The bacterial General Secretory System is centred around two essential components: the SecYEG complex, which forms a pore through the cytoplasmic membrane, and SecA, an ATPase that couples ATP binding and hydrolysis to translocation of an unfolded preprotein substrate through the SecYEG pore. Attempts to address this question have been confounded by the fact that SecA exists as a dimer in solution, but given the changes in SecA oligomerization required for its interaction with SecYEG, it is not clear whether the solution dimer is related to oligomeric species that may participate in the translocation reaction. Truncation of E. coli SecA at residue 610 produces a construct, SecA-N68, that is monomeric at low concentrations but at higher concentrations forms tetramers. In the current work, we have discovered that the formation of the SecA-N68 tetramer is completely dependent on unstructured polypeptide segments at its N- and C-termini.

To obtain a structure of the E. coli PPXD, we used a deletion construct, “SecA-N68” that lacks the C-terminal domains, including the Helical Wing Domain (HWD), the Helical Scaffold Domain (HSD), and a linker connected to the Zinc Binding Domain (ZBD). To obtain crystals of SecA-N68, we removed unstructured regions at the N- and C-termini so that the construct included residues 15 to 590, which we term “SecA-N68∆NC”. In addition, entropy-reducing mutations to alanine37 were introduced in two areas, one containing E55, K56, and E58, and a second at E196 and E197. In addition, removal of the termini allowed us to obtain crystals of SecA-N68 that diffracted to 2.6 Å resolution and yielded a structure that includes both the DEAD Motor domains and the preprotein crosslinking domain (PPXD), which was disordered in the original E. coli SecA structure. The structure of SecA-N68∆NC bound to Mg2+-ADP contains the DEAD Motor domains, NBD1 and NBD2, in the same conformation observed for other SecA structures, with the exception of the E. coli SecA structure which was crystallized in the absence of bound nucleotide and in which NBD1 and NBD2 adopt a more open conformation. The β-hairpin anchoring the PPXD to NBD1 is in a fully extended conformation that has not been observed in previous crystal structures, where the hairpin is typically bent to facilitate interaction of the PPXD with the C-terminal helical domains. The core PPXD structures are conserved throughout, with some differences in loop regions. Helix 4 is particularly well-conserved, likely because it plays a central role, interacting directly with SecYEG as well as Helix 1, 3, and Hairpin 2. That is, SecA-N68∆NC, in which both N- and C-termini had been truncated to remove unstructured polypeptide but is otherwise identical to SecA-N68, is completely monomeric when analyzed by gel filtration chromatography. Formation of the SecA-N68 tetramer is completely dependent on unstructured polypeptide at the N- and C-termini.

> GADRTLRRMRKVVNIINAMEPEMEKLSDEELKGKTAEFRARLAAGAVLENLIPEAFAVVREASKRVFGMRHFDVQLLGGMVLNERCIAEMRTGEGKTLTATLPAYLNALTGKGVHVVTVNDYLAQRDAENNRPLFEFLGLTVGINLPGMPAPAKREAYAADITYGTNNEYGFDYLRDNMAFSPAARVQRKLHYALVDEVDSILIDEARTPLIISGPAEDSSEMYKRVNKIIPHLIRQEKEDSETFQGEGHFSVDEKSRQVNLTERGLVLIEELLVKEGIMDEGESLYSPANIMLMHHVTAALRAHALFTRDVDYIVKDGEVIIVDEHTGRTMQGRRWSDGLHQAVEAKEGVQIQNENQTLASITFQNYFRLYEKLAGMTGTADTEAFEFSSIYKLDTVVVPTNRPMIRKDLPDLVYMTEAEKIQAIIEDIKERTAKGQPVLVGTISIEKSELVSNELTKAGIKHNVLNAKFHANEAAIVAQAGYPAAVTIATNMAGRGTDIVLGGSWQAEVAALENPTAEQIEKIKADWQVRHDAVLEAGGLHIIGTERHESRRIDNQLRGRSGRQGDAGSSRFYLSM> GSARQQEIDMKRQQRFFRIPFIRPADQYKDPQNKKKGWWYAHFDGPWIARQMELHPDKPPILLVAGKDDMEMCELNLEETGLTRKRGAEILPRQFEEIWERCGGIQYLQSAIESRQA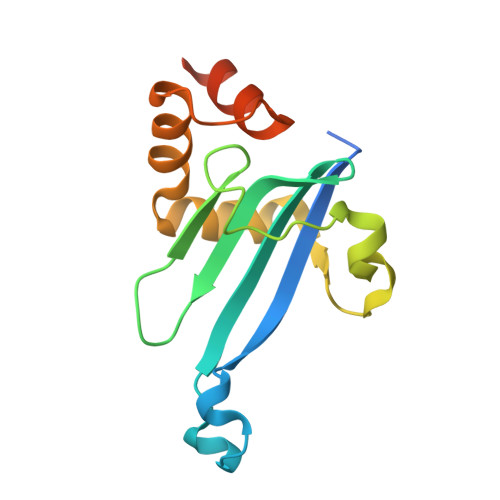RPTYATAMLQNLLKGSSGGSLVPR T-STAR is a tissue-specific STAR protein mainly expressed in the testis and brain3426, and regulates the alternative splicing of CD44, Tra2β, Tau, VGEF and Neurexin pre-mRNAs262728. STAR proteins are defined by the presence of a highly conserved RNA-binding domain, the STAR domain, also responsible for homodimerization, and composed of a central KH (K homology) domain flanked by two highly conserved regions, QUA1 and QUA2. Here, we have determined the X-ray structures of the T-STAR KH domain in its free state, and in complex with AAAUAA; KH-QUA2 in complex with AAUAAU; QUA1-KH in complex with UAAU; and the full STAR domain in complex with AUUAAA. Taken together, our data reveal a unique mode of RNA recognition and dimerization by the STAR proteins Sam68 and T-STAR that is crucial for their function in alternative splicing.

The KH domain of T-STAR adopts a classical type-I KH fold very similar to KH structures of other STAR proteins. A comparison of free and RNA-bound structures of T-STAR show that the presence of the QUA1, QUA2 and the RNA do not induce any global structural changes of the KH domain (backbone RMSD ranging between 0.44 and 1.05 Å). Surprisingly, the KH domain and the C-terminal half of the QUA1-KH linker of T-STAR provide an additional dimerization interface. This novel KH/linker interface covers 1,065 Å2 per monomer, almost twice as large as the QUA1 dimerization interface, and involves mainly the C-terminal α-helix 3 of the KH domain and the C-terminal half of the QUA1-KH linker. The KH interface is stabilized by a network of hydrophobic interactions involving residues A138, Y141, M144, G145 and L148, and an intermolecular hydrogen bond between Y141 in α-helix 3 and Q58 in β-strand 1 of the KH.

>[4x]GAINKNMKLGQKVLIPVKQFPKFNFVGKLLGPRGNSLKRLQEETLTKMSILGKGSMRDKAKEEELRKSGEAKYFHLNDDLHVLIEVFAPPAEAYARMGHALEEIKKFLIPDYN>[2x]MGFSLYTDDTVKAAAQYAYDNYLGKPYTGSVESAPANFGGRMVYRQHHGLSHTLRTMAYAELIVEEARKAKLRGETLGKFKDGRTIADVTPQELKKIMIAQAFFVAGRDDEASDAKNYQKYHEQSRDAFLKYVKDNESTLIPDVFKDQEDVNFYARVIEDKSHDWESTPAHVLINQGHMVDLVRVKQPPESFLQRYFSSMQRWIGSQATEAVFGIQRQFFHATYEVVAGFDSDNKEPHLVVSGLGRYVIGEDGQPIREAPKKGQKEGDLKVFPQTYKLKENERLMRVDEFLKLPEIQNTFPGSGKHLQGGMPGMNEMDYWNRLNSLNRARCENDVDFCLKQLQTAHDKAKIEPIKQAFQSSKGKERRQPNVDEIAAARIIQQILANPDC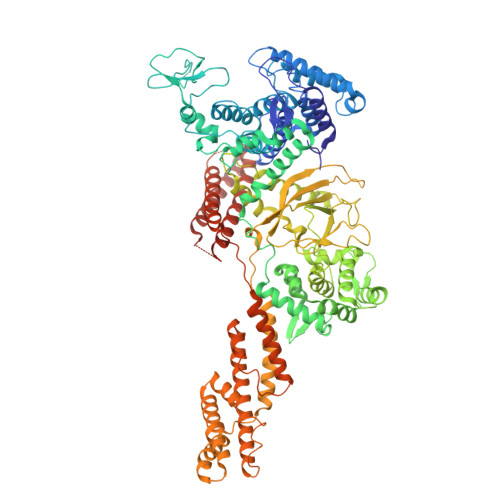IHDDHVLINGQKLEQQFFRDLLAKCEMAVVGSLLNDTDIGNIDTLMRHEKDTEFHSTNPEAVPVKIGEYWINDQRINNSSGNITQKKHDLIFLMQNDAWYFSRVNAIAQNRDKGSTFKEVLITTLMTPLTSKALVDTSQAKPPTRLFRGLNLSEEFTKGLIDQANAMIANTTERLFTDHSPEAFKQIKLNDLSKMSGRTNASTTTEIKLVKETWDSNVIFEMLDPDGLLHSKQVGRHGEGTESEFSVYLPEDVALVPVKVTLDGKTQKGENRYVFTFVAVKSPDFTPRHESGYAVEPFLRMQAAKLAEVKSSIEKAQRAPDLETIFNLQNEVEAVQYSHLSTGYKNFLKNTVGPVLENSLSGLMESDTDTLSKALAAFPSDTQWSAFNFEEARQAKRQMDAIKQMVGNKVVLDALTQCQDALEKQNIAGALDALKKIPSEKEMGTIRRELREQIQSARQELESLQRAVVTPVVTDEKKVRERYDALIENTSKKITELETGKLPNLDAVKKGISNLSNLKQEVTVLRNEKIRMHVGTDKVDFSDVEKLEQQIQVIDTKLADAYLLEVTKQIS> MTAVADAPQADIEGVASPQAVVVGVMAGEGVQIGVLLDANAPVSVMTDPLLKVVNSRLRELGEAPLEATGRGRWALCLVDGAPLRATQSLTEQDVYDGDRLWIRFIADTERRSQVIEHIST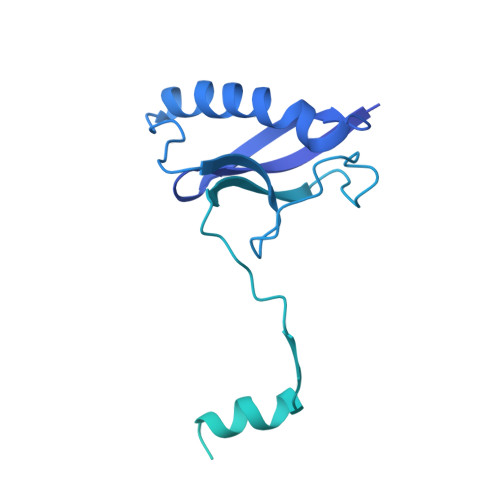AVASDLSKRFARIDPIVAVQVGASMVATGVVLATGVLGWWRWHHNTWLTTIYTAVIGVLVLAVAMLLLMRAKTDADRRVADIMLMSAIMPVTVAAAAAPPGPVGSPQAVLGFGVLTVAAALALRFTGRRLGIYTTIVIIGALTMLAALARMVAATSAVTLLSSLLLICVVAYHAAPALSRRLAGIRLPVFPSATSRWVFEARPDLPTTVVVSGGSAPVLEGPSSVRDVLLQAERARSFLSGLLTGLGVMVVVCMTSLCDPHTGQRWLPLILAGFTSGFLLLRGRSYVDRWQSITLAGTAVIIAAAVCVRYALELSSPLAVSIVAAILVLLPAAGMAAAAHVPHTIYSPLFRKFVEWIEYLCLMPIFPLALWLMNVYAAIRYR>[6x]MAGSELRAELEQRLGALAIRTEVVEHPEVFTIEEMMPHIQHLKGAHSKNLFLKDKKKKNYWLVTVLHDRQINLNDLGKQLGVGSGNLRFADETAMLEK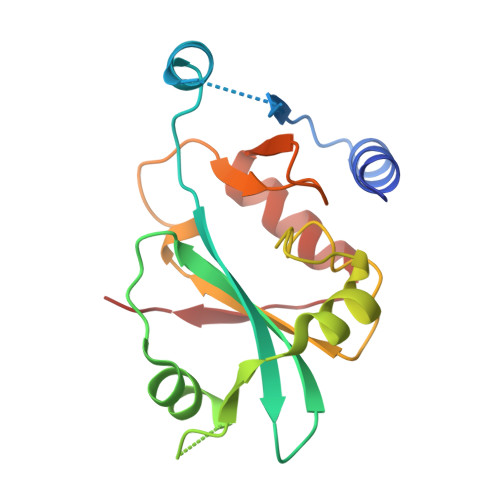LKVGQGCATPLSLFCDDGDVKFVLDSAFLEGGHEKVYFHPMTNAATMGLSPEDFLIFVKATGHDPIILNFD In particular, evasins (designated by the prefix “EVA”) are produced in the saliva of ticks and bind to chemokines, thus preventing chemokine receptor activation and the downstream inflammatory cascade (Bhusal et al., 2020). Evasins belonging to class A bind exclusively to CC chemokines, whereas those belonging to class B bind exclusively to CXC chemokines. We recently described class A3 evasins, which have 10 cysteines and an additional disulfide, and reported chemokine‐bound structures of the class A3 evasin EVA‐AAM1001 (Devkota et al., 2023). We now describe a structure–function analysis of EVA‐ACA1001, a class A3 evasin from Amblyomma cajennense (Cayenne tick).

To understand how the core of EVA‐ACA1001 defines broad‐spectrum binding, we determined the crystal structure of EVA‐ACA1001 in complex with the human chemokine CCL16 to a resolution of 2.7 Å resolution. The complex crystallized in 1:1 stoichiometry with two molecules per asymmetric unit. In both complexes, the extreme N‐ and C‐termini of both EVA‐ACA1001 and CCL16 were not clearly visible in the electron density maps, consistent with the minimal contributions of these regions to binding. EVA‐ACA1001 comprises one β‐strand forming an anti‐parallel beta sheet with the CC motif of CCL16, two antiparallel β‐sheets, and two α‐ helices. As expected, the structure contains five intramolecular disulfide bonds, four (Cys27‐Cys49, Cys45‐Cys86, Cys62‐Cys91, and Cys81‐Cys100) of which are conserved in all class A evasins, and the fifth (Cys25‐Cys54) that is unique to class A3 evasins. EVA‐ACA1001 interacts with the chemokine CC motif, the residue immediately following the CC motif (“CC + 1” residue), and a shallow groove between the N‐loop and the third β‐strand (β3). The CC motif of CCL16 interacts with EVA‐ACA1001 through four backbone‐backbone hydrogen bonds. The CC + 1 residue (Leu19) of CCL16 is located within a deep hydrophobic pocket in the core of EVA‐ACA1001. The hydrophobic pocket is defined by the side chains of Cys27, Ala29, Pro30, His31, Pro42, Tyr47, Cys49, Pro57, and Tyr60 and by the Cys25–Cys54 disulfide bond, the unique disulfide in class A3 evasins. Notably, His31, Pro42, and Tyr60 form a hydrophobic cluster at the base of the hydrophobic pocket, which differs from the equivalent region of EVA‐AAM1001 and may contribute to the broader spectrum of chemokine binding by EVA‐ACA1001 (see Discussion).

>[2x]ENGEGTTQPDYDNSTDYYNYEDFKCTCPAPHLNNTNGTVMKPIGCYYTCNVTRCTAPDTYPCYNLTEHQAKNLTTSPTTLCAVGNCDHGICVPNGTKELCFKAPNLEE;>GPSQPKVPEWVNTPSTCCLKYYEKVLPRRLVVGYRKALNCHLPAIIFVTKRNREVCTNPNDDWVQEYIKDPNLPLLPTRNLSTVKIITAKNGQPQLLNSQ[2x]>[4x]SNAMKWLEESIMVKRGVGAGRKPVTHHLTEEMQKEFHYTIGPYSTPVLTIEPGDRVIVDTRDAFEGAISSEQDIPSQLLKMPFLNPQNGPIMINGAEKGDVIAVYIESMLPRGVNPHGICAMIPHFGG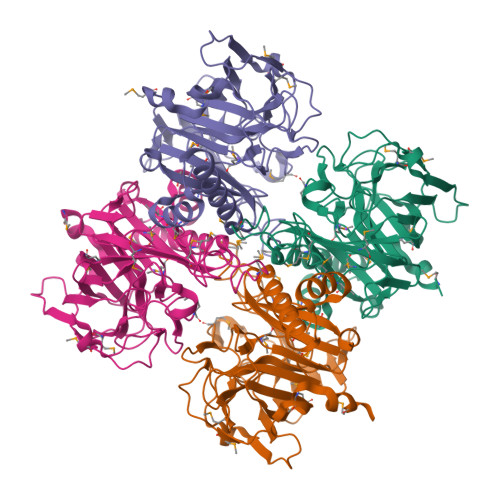LTGTDLTAMLNDPLPEKVRMIKLDSEKVYWSERHTLPYKPHIGTLSVSPEIDSINSLTPDNHGGNMDVPDIGPGSITYLPVRAPGGRLFIGDAHACQGDGEICGTAVEFASITTIKVDLIKNWQLSWPRMENAETIMSIGSARPLEDATRIAYRDLIYWLVADFGFEQWDAYMLLSQCGKVRLGNMVDPKYTVGAMLNKELLAQ>GAASKKVNVLVVGLDNSGKTTIIERLKPRPRQAAEVAPTVGFTVDEVEKGPLTFTVFDMSGAGRYRTLWEQYYREADAVVFVVDSADKLRMVVARDEMEHMLKHSNMRKVPILYFANKKDLPVAMPPVEIAQALGLDDIKDRPWQIVPSNGLTGEGVDKGIDWLAERLS[3x];>[4x]MVHESNPNDYAAGDAGNASGRYTTGSNGIPPMLPSVRSVWLDAFNDPVAGISAYTPCVHTCNLFGDGENRLVIADEDRKLKIWKGTQKASEHPLLDTPVAICSYISENTAPRLPALAVAAGSHIYIYRNLRPYYKFVLPPENVNTEEQDIWQKVMEGEIVIGEAVAQLTRLQVRAGDAGVVLQTRSLQLMNIGDPDAKMAFVEHWQGQPLVATTVITCMDVVKQAIDEPDAVSCLVVGTESGRILILNPAGTAIVKNIWVGITPAMIAVQGELDVGYRITVAGRDGKLYHIRNGELSQTIIQLEAQPVGL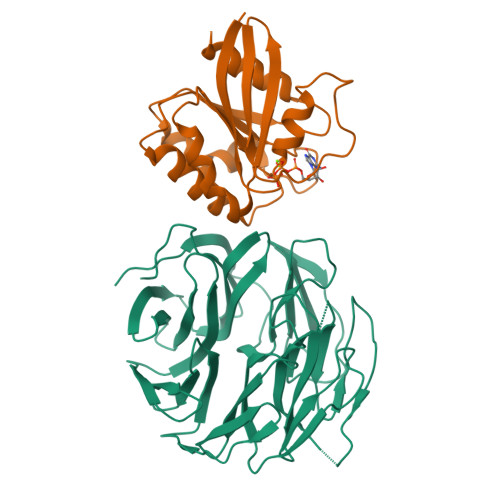VRLAKHVAVGCMNDVVHAYTPTGHKSWSLYLPCHILAMQRMEVTGQRNTKALIVALSNGEVRVYNEKLLVSVHVSPNPVTALWFGRYGREDNTLLAITKSGALDIKMLPRTANLE;> GAASKKVNVLVVGLDNSGKTTIIERLKPRPRQAAEVAPTVGFTVDEVEKGPLTFTVFDMSGAGRYRTLWEQYYREADAVVFVVDSADKLRMVVARDEMEHMLKHSNMRKVPILYFANKKDIPVAMPPVEIAQALGLDDIKDRPWQIVPSNGLTGEGVDKGIDWLAERLS> VKLAGNSSLCPINGWAVYSKDNSIRIGSKGDVFVIREPFISCSHLE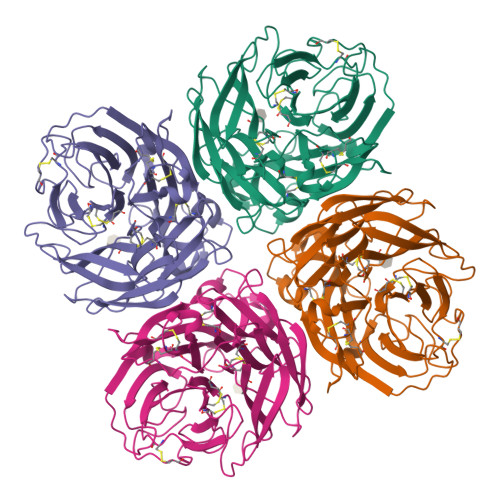CRTFFLTQGALLNDKHSNGTVKDRSPHRTLMSCPVGEAPSPYNSRFESVAWSASACHDGTSWLTIGISGPDNGAVAVLKYNGIITDTIKSWRNNILRTQESECACVNGSCFTVMTDGPSNGQASYKIFKMEKGKVVKSVELDAPNYYYEECSCYPNAGEITCVCRDNWHGSNRPWVSFNQNLEYQIGYICSGVFGDNPRPNDGTGSCGPVSSNGAYGVKGFSFKYGNGVWIGRTKSTNSRSGFEMIWDPNGWTETDSSFSVKQDIVAITDWSGYSGSFVQHPELTGLDCIRPCFWVELIRGRPKESTIWTSGSSISFCGVNSDTVGWSWPDGAELPFTI>[4x]VVLRVVTVLEEPFVMVSENVLGKPKKYQGFSIDVLDALSNYLGFNYEIYVAPDHKYGSPQEDGTWNGLVGELVFKRADIGISALTITPDRENVVDFT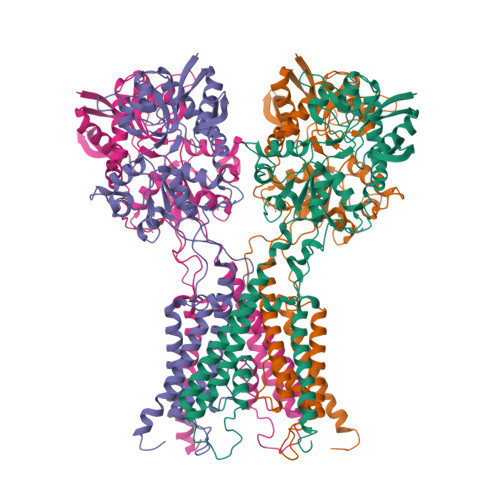TRYMDYSVGVLLRRAEKTVDMFACLAPFDLSLWACIAGTVLLVGLLVYLLNWLNPPRLQMGSMTSTTLYNSMWFVYGSFVQQGGEVPYTTLATRMMMGAWWLFALIVISSYTANLAAFLTITRIESSIQSLQDLSKQTEIPYGTVLDSAVYEHVRMKGLNPFERDSMYSQMWRMINRSNGSENNVLESQAGIQKVKYGNYAFVWDAAVLEYVAINDPDCSFYTIGNTVADRGYGIALQHGSPYRDVFSQRILELQQNGDMDILKHKWWPKNGQCDLYSSVDTKQKGGALDIKSFAGVFCILAAGIVLSCFIAMLETWWNKRKGSR>DKATIPSESPFAAAEVADGAIVVDIAKMKYETPELHVKVGDTVTWINREAMPHNVHFVAGVLGEAALKGPMMKKEQ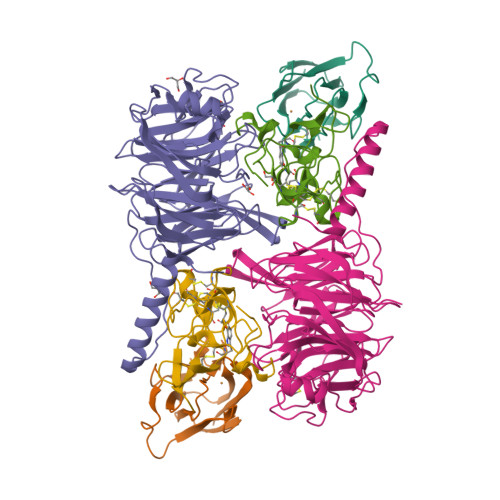AYSLTFTEAGTYDYHCTPHPFMRGKVVVE[2x];>QDAPEAETQAQETQGQAAARAAAADLAAGQDDEPRILEAPAPDARRVYVNDPAHFAAVTQQFVIDGEAGRVIGMIDGGFLPNPVVADDGSFIAHASTVFSRIARGERTDYVEVFDPVTLLPTADIELPDAPRFLVGTYPWMTSLTPDGKTLLFYQFSPAPAVGVVDLEGKAFKRMLDVPDCYHIFPTAPDTFFMHCRDGSLAKVAFGTEGTPEITHTEVFHPEDEFLINHPAYSQKAGRLVWPTYTGKIHQIDLSSGDAKFLPAVEALTEAERADGWRPGGWQQVAYHRALDRIYLLVDQRDEWRHKTASRFVVVLDAKTGERLAKFEMGHEIDSINVSQDEKPLLYALSTGDKTLYIHDAESGEELRSVNQLGHGPQVITTADMG[2x];>ADAPAGTDPRAKWVPQDNDIQACDYWRHCSIDGNICDCSGGSLTNCPPGTKLATASWVASCYNPTDGQSYLIAYRDCCGYNVSGRCPCLNTEGELPVYRPEFANDIIWCFGAEDDAMTYHCTISPIVGKAS[2x]2-BROMOPHENOL | C6 H5 Br O | 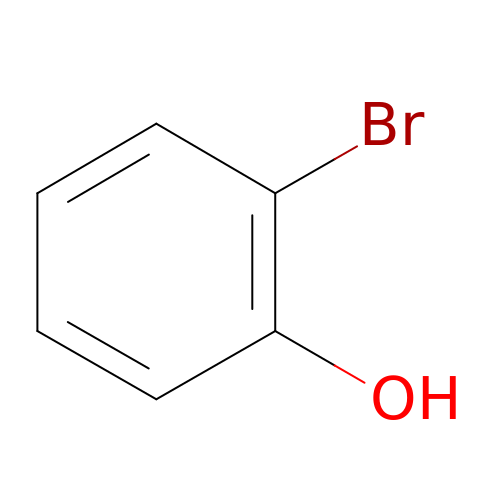VADKRMSMGWJZCF-UHFFFAOYSA-N> TSNEVAQFLSKENQVIVRMRGLPFTATAEEVVAFFGQHCPITGGKEGILFVTYPDGRPTGDAFVLFACEEYAQNALRKHKDLLGKRYIELFRSTAAEVQQVLN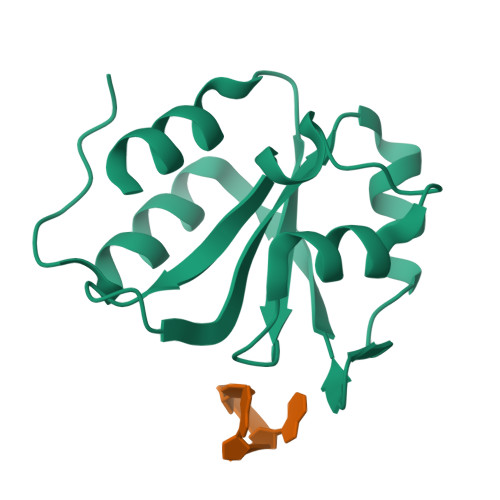RFSSAPLIPLPTPPII> MTGSTSHITILTLNINGLNSAIKRHRLASWIKSQDPSVCCIQETHLTCRDTHRLKIKGWRKIYQANGKQKKAGVAILVSDKTDFKPTKIKRDKEGHYIMVKGSIQQEELTILNIYAPNTGA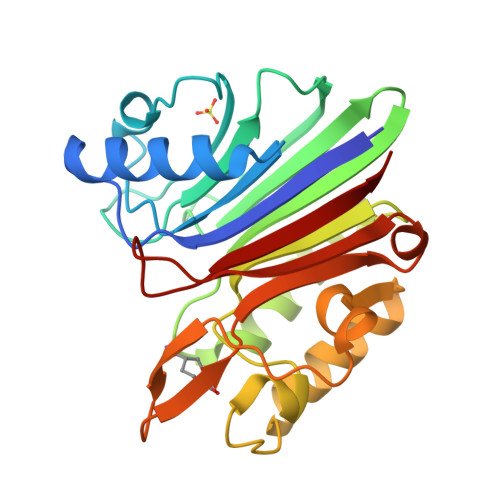PRFIKQVLSDLQRDLDSHTLIMGDFNTPLSTLDRSTRQKVNKDTQELNSALHQADLIDIYRTLHPKSTEYTFFSAPHHTYSKIDHIVGSKALLSKCKRTEIITNYLSDHSAIKLELRI(3~{S},4~{S},5~{R})-4-acetamido-3-oxidanyl-5-[(1~{S},2~{R})-1,2,3-tris(oxidanyl)propyl]cyclohexane-1-carboxylic 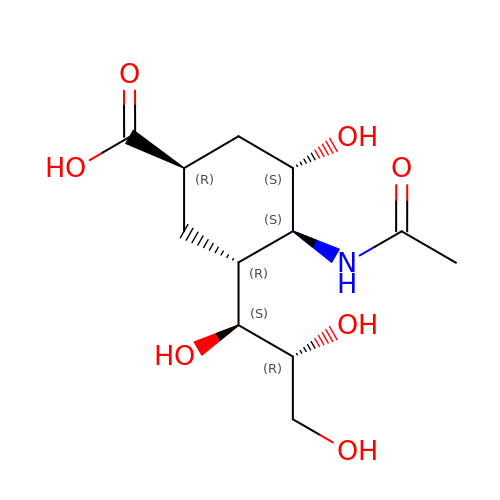acid | C12 H21 N O7 | DHTDKODYGURRPR-UUFBCVLASA-N> GASGDLYEVERIVDKRKNKKGKWEYLIRWKGYGSTEDTW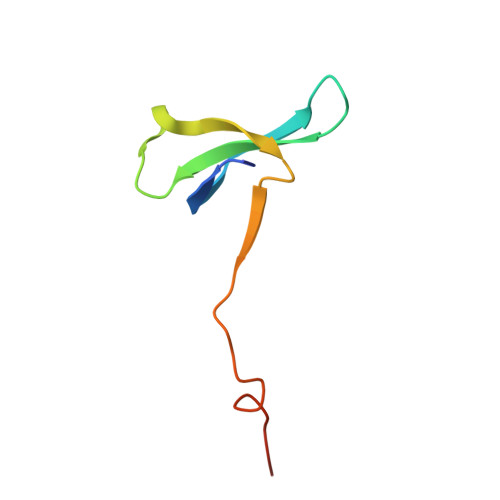EPEHHLLHCEEFIDEFNGLHMSKDK>GSHMTPNKEDYLKCIYEIGEQEPKITNKMVAEKMHVSAPAVSEMIKKMISQGWIVKDKAKGYLLKDKGYALVANLYRKHRLIEVFLIHQLGYNTQEVHQEAEVLEHTVSDTFIDRLDKILDFPDFCPHGGTIPRYGQPLVEMNT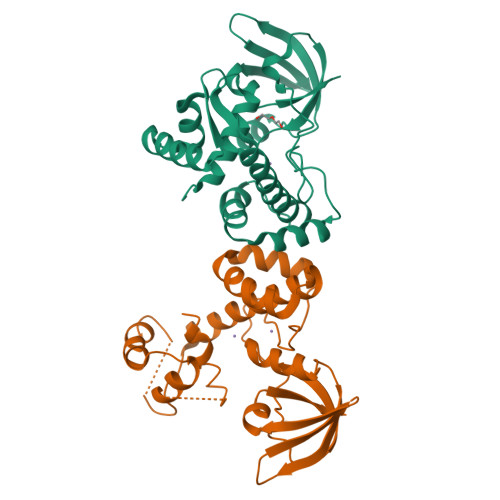TTLNTITELGRFRLSRIHDHFDLIQYLETHHLNINTELTLTQIDTFAKTYTICYGDKELVIPENIAKQLYVTAL[2x]> MEKVFYVTTPIYYVNAEPHLGHAYTTVVADFLARWHRLDGYRTFFLTGTDEHGETVYRAAQAAGEDPKAFVDRVSGRFKRAWDLLGIAYDDFIRTTEERHKKVVQLVLKKVYEAGDIYYGEYEGLYCV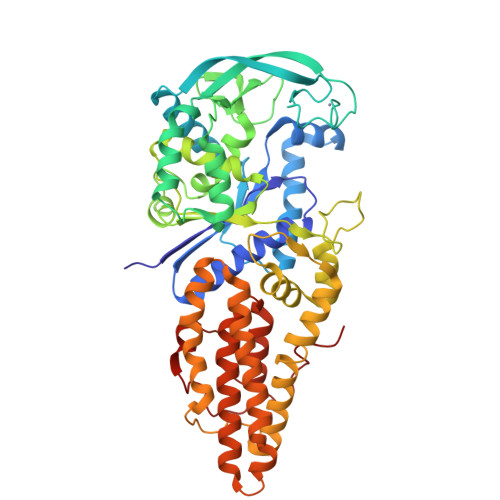SCERFYTEKELVEGLCPIHGRPVERRKEGNYFFRMEKYRPWLQEYIQENPDLIRPEGYRNEVLAMLAEPIGDLSISRPKSRVPWGIPLPWDENHVTFVWFDALLNYVSALDYPEGEAYRTFWPHAWHLIGKDILKPHAVFWPTMLKAAGIPMYRHLNVGGFLLGPDGRKMSKTLGNVVDPFALLEKYGRDALRYYLLREIPYGQDTPVSEEALRTRYEADLADDLGNLVQRTRAMLFRFAEGRIPEPVAGEELAEGTGLAGRLRPLVRELKFHVALEEAMAYVKALNRYINEKKPWELFKKEPEEARAVLYRVVEGLRIASILLTPAMPDKMAELRRALGLKEEVRLEEAERWGLAEPRPIPEEAPVLFPKK>[2x]KMNESDIWFEEKLQEVECEEQRLRKLHAVVETLVNHRKELALNTAQFAKSLAMLGSSEDNTALSRALSQLAEVEEKIEQLHQEQANNDFFLLAELLSDYIRLLAIVRAAFDQRMKTWQRWQDAQATLQKKREAEARLLWANKPDKLQQAKDEILEWESRVTQYERDFERISTVVRKEVIRFEKEKSKDFKNHVIKYLETL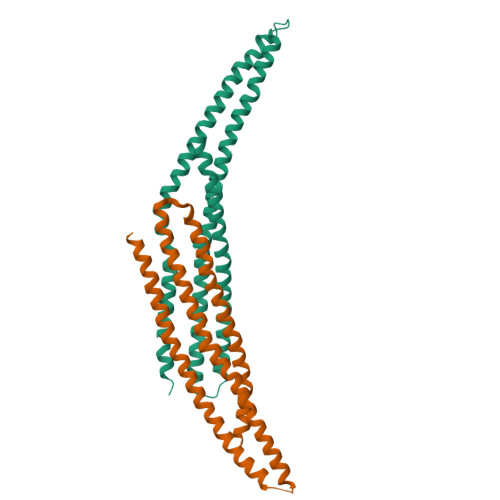LYSQQQLAKYWEAFLPEAKAIS;>[2x]DEVLFTGVKEVDDFFEQEKNFLINYYNRIKDSCVKADKMTRSHKNVADDYIHTAACLHSLALEEPTVIKKYLLKVAELFEKLRKVEGRVSSDEDLKLTELLRYYMLNIEAAKDLLYRRTKALIDYENSNKALDKARLKSKDVKLAEAHQQECCQKFEQLSESAKEELINFKRKRVAAFRKNLIEMSELEIKHARNNVSLLQSCIDLFKNN>AMTDIPDRKEAVISLWPEFAKAIVSGKKTVEFRRRIPLPALSARIWIYATRPVKSVIGFAYLEAIVQGDVNTLWSRYGREAFLSEQQYRDYFEGTEKATAFLLRDHQPIRPINLDQLKEIRANFQPPQALTWLRKEETQKLVSLTSQVE[2x]

In the ethanologenic bacterium Zymomonas mobilis ZM4, the gene ZMO0922 encodes a 148 amino acid polypeptide, which has been annotated as a putative ASCH domain-containing protein (ZmASCH) that belongs to family 23. Here, we report the three-dimensional crystal structure of ZmASCH which confirms the fold of a central β-barrel core and reveals a positively-charged cleft with a pocket on the surface. In vitro assays showed that ZmASCH bound nucleic acids and possessed cleavage activity specifically towards single-stranded RNAs. The weak nuclease activity of ZmASCH depended on magnesium ions and the protein appeared to prefer the consecutive pyrimidine-adenine dinucleotides for its cleavage activity.

The bases of the bound ssRNA interact with the side-chain atoms of Arg32, Tyr90, Lys117, Gln124, and Ser128. Although these residues are not conserved in ZmASCH at the same site, potential polar residues (Asn122, Gln124, Gln127, and Ser128), which might possibly interact with RNA molecules, are found nearby (right). Based on these simulation results and extensive analysis of amino acid sequences of related proteins, we introduced a charge-reversal mutation at the site of Lys53 (K53E), within the positively charged surface cleft. This mutant exhibited reduced binding to ssDNA and ssRNA molecules. Another mutation at Ser128 (S128A) also decreased the binding of ZmASCH to nucleic acids, although to a lesser degree. Mutations of the two independent residues at the positions of 47 and 128 did not make a noticeable structural change.> QTGGSFFEPFNSYNSGTWEKADGYSNGGVFNCTWRANNVNFTNDGKLKLGLTSSAYNKFDCAEYRSTNIYGYGLYEVSMKPAKNTGIVSSFFTYTGPAHGTQWDEIDIEFLGKDTTKVQFNYYTNGVGGHEKV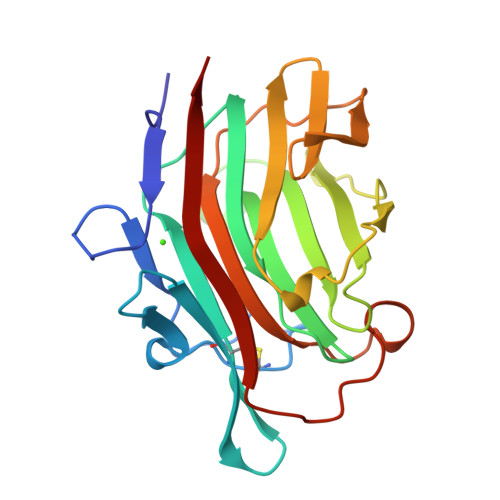ISLGFDASKGFHTYAFDWQPGYIKWYVDGVLKHTATANIPSTPGKIMMNLWNGTGVDDWLGSYNGANPLYAEYDWVKYTSN>[4x]MGSSHHHHHHSSGRENLYFQGMTKMNRETVITEALDLLDEVGL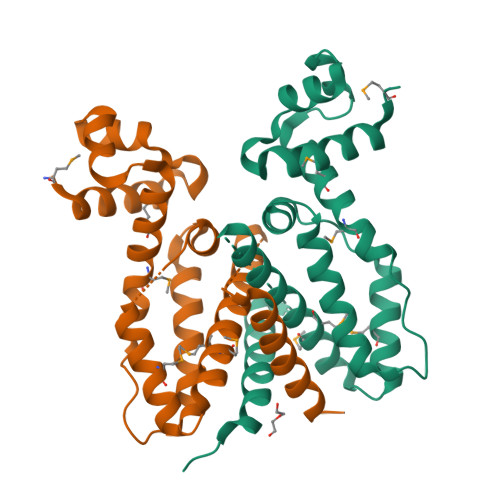DGVSTRRLAKRLGVEQPSLYWYFRTKRDLLTAMAQAAMAPHAAEPLPEPGEDWHGWFLRNTRSFRRTLLARRDGARLHAGSRPTADLDRVRRKMDFLVASGVPERHAQMAMLAAGRFTVGCVLEEQAETGAGDTADLPADVPEIDHESAFEAGLALITDGLVRHVDAR>VQIHDITGKDCQDIANKGAKQSGLYFIKPLKANQQFLVYCEIDGSGNGWTVFQKRLDGSVDFKKNWIQYKEGFGHLSPTGTTEFWLGNEKIHLISTQSAIPYALRVELEDWNGRTSTADYAMFKVGPEADKYRLTYAYFAGGDAGDAFDGFDFGDDPSDKFFTSHNGMQFSTWDNDNDKFEG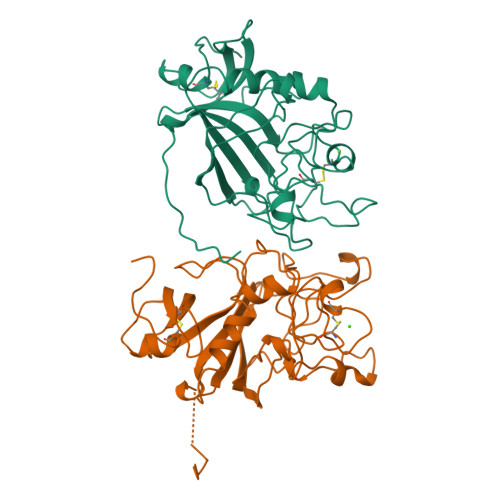NCAEQDGSGWWMNKCHAGHLNGVYYQGGTYSKASTPNGYDNGIIWATWKTRWYSMKKTTMKIIPFNRLTIGEGQQHHLGGAKQAGDV[2x]>MDEAPETTTASPAAQVLEGKTMGTLWRVSVVGIDAKRAAELQTKIQTQLDADDWLLSTYKNDSALMRFNHSRSLAPWPVSEAMADIVTSALRIGAKTDGAMDITVGPLVNLWGFGPDRQPLHIPTPAQIDAAKAKTGLQHLQVIDRAGHQFLQKDLPDLYVDLSTVGEGYAADHLARLMEQEGIARYLVSVGGALSSRGMNAQGQPWRVAIQKPTDRENAVQAIVDINGHGISTSGSYRNYY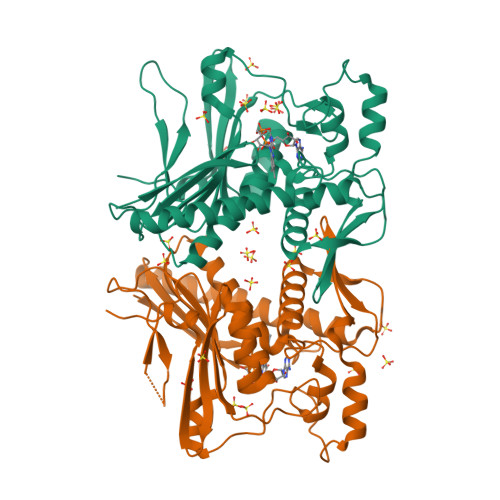ELDGKRVSHVIDPQTGRPIEHNLVSVTVIAPTALEADGWDTGLMVLGTQKAQEVVRREGLAVFMIMKEGEGFKTWMSPQFKTFLVSDKNHHHHHH[4x]>[2x]MVARVQTAEEIRDEGNAAVKDQDYIKADELYTEALQLTTDEDKALRPVLYRNRAMARLKRDDFEGAQSDCTKALEFDGADVKALFRRSLAREQLGNVGPAFQDAKEALRLSPNDKGIVEVLQRLVKANNDKIKQTTSLANKVTDMEKLAFRGEAKDTEQKMTALNNLLVLCRESESGATGVWNQGALVPFVLNLINDASENEEVTVTAIRILDETIKNSVRCMKFLAMHDPDGPKSVRFVCRLMCKKSTKDFVDATGILVQRVFNAMAKMDRQKEMKPDPEVAEANKIWIIRVLLELQEMLQDPKVGAVQRETCIDLFLKNLMHMDGGIPRGWSWKFVEERGLLALLDVASQIPELCEYPVSAETRQHVAICLQRLEEDMVFDTKRTIFKEKVDMFFNALISRCTNDDEGHKYRIKLSCFLITMLQGPVDIGINLITNDQLTPIMLEMAASQDHLMQGIAAELIVATVSKHERAINMLKVGIPVLRALYDSEDPTVKVRALVGLCKIGAAGGDDISKATMKEEAVISLAKTCKKFLLETEKYSVDIRRYACEGLSYLSLDADVKEWIVDDSLLLKALVLLAKKAGALCVYTLATIYANLSNAFEKPKVDEEMVKLAQFAKHHVPETHPKDTEEYVEKRVRALVEEGAVPACVAVSKTESKNALELIARSLLAFAEYEDLRGRIIAEGGTVLCLRLTKEASGEGKIKAGHAIAKLGAKADPMISFPGQRAYEVVKPLCDLLHPDVEGKANYDSLLTLTNLASVSDSIRGRILKEKAIPKIEEFWFMTDHEHLRAAAAELLLNLLFFEKFYEETVAPGTDRLKLWVLYSAEVEEERLSRASAAGFAILTEDENACARIMDEIKSWPEVFKDIAMHEDAETQRRGLMGIANIMHSSNKLCSEIVSSEVFRVLVAVTKLXXXXXXXXXXXXXXXXXXXXXXXXXXXXXXXXXXXXXXXXXXXXXXXX

Subsequent studies in C. elegans, Xenopus, Zebrafish, and Drosophila confirmed the role of UNC-45 as a myosin-specific chaperone, promoting the folding of the myosin ATPase domain as well as coordinating the assembly of thick filaments during muscle development. To better understand its myosin folding function, we established an orthogonal protein folding assay in insect cells, characterizing the interplay of the C. elegans muscle myosin MHC-B with its cognate chaperone UNC-45. Structural data of various functional mutants clarify the role of the distinct UNC-45 domains in this process providing important mechanistic insight into its myosin folding activity.

Surprisingly, however, deleting the entire TPR domain fully abolished the chaperone function of UNC-45. Accordingly, the TPR domain does not only serve as Hsp70/Hsp90 docking site, but accomplishes further critical functions. Finally, we determined the crystal structure of the UNC-45 ∆TPR construct that represents a C. elegans UNC-45 variant in monomeric, non-filamentous form. The asymmetric unit of the ∆TPR crystal form is built up by two molecules. In molecule A, the UCS domain adopts an extended conformation similar to wt UNC-45, whereas molecule B contains a UCS domain that is strongly bent, with the entire domain and even more strongly its C-terminal half (ARM repeats 14–17) extending away from the central domain. These data further highlight the pronounced structural flexibility of the myosin-binding UCS domain, which is held in place by non-covalent interactions with the adjacent central and TPR domains. Accordingly, deleting the TPR domain releases the flexible UCS domain to adopt various conformations, two of which were captured in the present crystal form. (2) Our structural data suggest that the TPR domain obtains an additional intra-molecular scaffolding role. It undergoes van-der-Waals contacts with the UCS domain, thereby arranging the myosin binding site to accommodate substrate. Our structural data reveal the capability of the UCS domain to adopt distinct defined conformations. Together, the wt, G427E, L822F, and ∆TPR crystal structures depict four different UCS conformations highlighting the pronounced dynamicity of the myosin-binding domain.> GSHMKPEIKEAYMKTAELFSQVSNCKRMKVGAIVVKNGSILAHGWNGTPSGFHTNCCELEDGSTNPFVLHAEQNA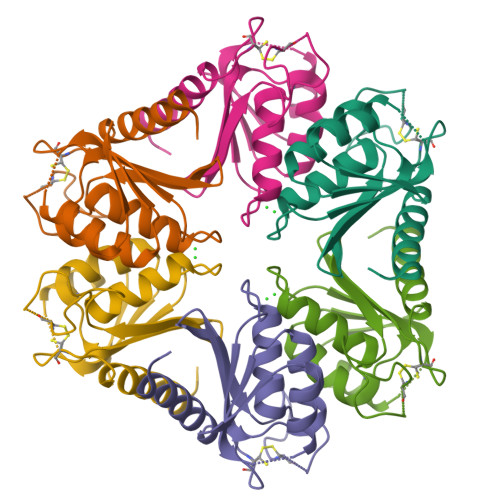LVKMAKSSESIDGSELFCTHSPCPDCSKMIAQAGVKKVYYRNEYRITDGIDVLQQLGVEVEKM> AGLVPRGSHMMEILRGSPALSAFRINKLLARFQAANLQVHNIYAEYVHFADLNAPLNDSEQAQLTRLLQYGPALSSHTPAGKLLLVTPRPGTISPWSSKATDIAHNCGLQQVDRLERGVAYYIEASTLTAEQWRQVAAELHDRMMETVFSSLTDAEKLFIHHQPAPVSSVDLLGEGRQALIDANLRLGLALAEDEIDYLQEAFTKLGRNPNDIELYMFAQANSEHCRHKIFNADWIIDGKPQPKSLFKMIKNTFETTPDYVLSAYKDNAAVMEGSAVGRYFADHNTGRYDFHQEPAHILMKVETHNHPTAISPWPGAATGSGGEIRDEGATGRGAKPKAGLVGFSVSNLRIPGFEQPWEEDFGKPERIVTALDIMTEGPLGGAAFNNEFGRPALTGYFRTYEEKVNSHNGEELRGYHKPIMLAGGIGNIRADHVQKGEIVVGAKLIVLGGPAMNIGLGGGAASSMASGQSDADLDFASVQRDNPEMERRCQEVIDRCWQLGDANPILFIHDVGAGGLSNAMPELVSDGGRGGKFELRDILSDEPGMSPLEIWCNESQERYVLAVAADQLPLFDELCKRERAPYAVIGDATEEQHLSLHDNHFDNQPIDLPLDVLLGKTPKMTRDVQTLKAKGDALNRADITIADAVKRVLHLPTVAEKTFLVTIGDRTVTGMVARDQMVGPWQVPVADCAVTTASLDSYYGEAMSIGERAPVALLDFAASARLAVGEALTNIAATQIGDIKRIKLSANWMAAAGHPGEDAGLYDAVKAVGEELCPQLGLTIPVGKDSMSMKTRWQEGNEQREMTSPLSLVISAFARVEDVRHTLTPQLSTEDNALLLIDLGKGHNALGATALAQVYRQLGDKPADVRDVAQLKGFYDAMQALVAARKLLAWHDRSDGGLLVTLAEMAFAGHCGVQVDIAALGDDHLAALFNEELGGVIQVRAEDRDAVEALLAQYGLADCVHYLGQALAGDRFVITANDQTVFSESRTTLRVWWAETTWQMQRLRDNPQCADQEHEAKANDTDPGLNVKLSFDINEDIAAPYIATGARPKVAVLREQGVNDHVEMAAAFHRAGFDAIDVHMSDLLGGRIGLGNFHALVACGGFSYGDVLGAGEGWAKSILFNHRVRDEFETFFHRPQTLALGVCNGCQMMSNLRELIPGSELWPRFVRNHSDRFEARFSLVEVTQSPSLLLQGMVGSQMPIAVSHGEGRVEVRDDAHLAALESKGLVALRYVDNFGKVTETYPANPNGSPNGITAVTTENGRVTIMMPHPERVFRTVANSWHPENWGEDSPWMRIFRN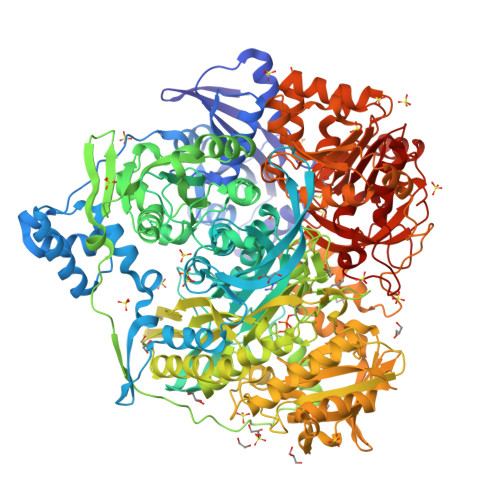ARKQLG> GGSGNEPTQEKHFMVYYRAWRDKTMQGVNTTLPDENWLTMHDIPYGIDIVNVFSYVPKGQEALAQPFYDTLKNEYAPALHARGVRLVRGIDYSELLKVPYAGTTPTEAEFDAYAKELLTKFVDDLGIDGLDIDMETRPSEKDIVLSNGVIRALSKYIGPKSGTDRPFLYDTNAEYLPPLQDVSDCFDFLAYQQYGSDDKRTQRALNNLSPVLNGERFVPGLTFPEEQDRNRWYDTKEPYMESNMYKVARYSYENNLGGMFLYALDRDGRTYNEDDLNQIKPSNLLWTKTAIAESKGVSLAEMKAAAQHYLKRISYANTDLEAQNKAAETVTQATTLYDVNKAILGGDYGQGLSNTYDAELEKGLLAIDLTTLYRALDQAVAAIEKAESYTPETIQALQTTKESVATELAGKTYTAAQVTTWQTEVQTALDNLKEK

Here we focus on EndoE, a multi-modular glycoside hydrolase secreted by Enterococcus faecalis, one of the leading causes of healthcare-associated infections. We provide X-ray crystal structures of EndoE, which show an architecture composed of four domains, including GH18 and GH20 glycoside hydrolases connected by two consecutive three α-helical bundles. We determine that the GH20 domain is an exo-β-1,2-N-acetylglucosaminidase, whereas the GH18 domain is an endo-β-1,4-N-acetylglucosaminidase that exclusively processes the central core of complex-type or high-mannose-type N-glycans. Both glycoside hydrolase domains act in a concerted manner to process diverse N-glycans on glycoproteins, including therapeutic IgG antibodies.

EndoE-GH18L crystallized in the P 6 5 space group with one molecule in the asymmetric unit and diffracted to a maximum resolution of 1.7 Å. The high quality of the electron density maps allowed us to trace residues 61–482. The GH18 domain (residues 61–349) adopts the conserved (β/α)8-barrel topology with an overall size of 45 × 46 × 38 Å. A large groove contains the active site. This groove is located at the center of the (β/α)8-barrel and surrounded by the loops connecting β1–α1 (loop 1; residues 70–90, pink), β2–α2 (loop 2; residues 105–111, brown), β3–α3 (loop 3; residues 143–157, orange), β4–α4 (loop 4; residues 185–190, light green), β5–α5 (loop 5; residues 223–227, blue), β6–α6 (loop 6; residues 244–248, green), β7–α7 (loop 7; residues 274–293, light blue), and β8–α8 (loop 8; residues 314–335, red). The floor of this groove is composed of a set of aromatic residues including Y67, W71, F104, Y245, and Y313. The crystal structure of the EndoE-GH18L construct revealed that the linker region folds into two three α-helical bundle (3HB) domains connected by an additional α-helix. The first 3HB domain comprises helices α9, α10 and α11 (3HB-1; residues 350–395), whereas the second 3HB domain covers helices α13, α14, and α15 (3HB-2; residues 421–482). Both 3HB-1 and 3HB-2 domains are connected by a short α-helix, α12 (residues 409–417). The GH18 and 3HB-1 domains interact with each other through an extensive contact area of ca. 972 Å2, representing 7% of the total accessible surface of the isolated domains.> GSHMADPDVLTEVPAALKRLAKYVIRGFYGIEHALALDILIRNSCVKEEDMLELLKFDRKQLRSVLNNLKGDKFIKCRMRVETAADGKTTRHNYYFINYRTLVNVVKYKLDHMRRRIETDERDSTNRASFKCPVCSSTFTDLEANQLFDPMTGTFRCT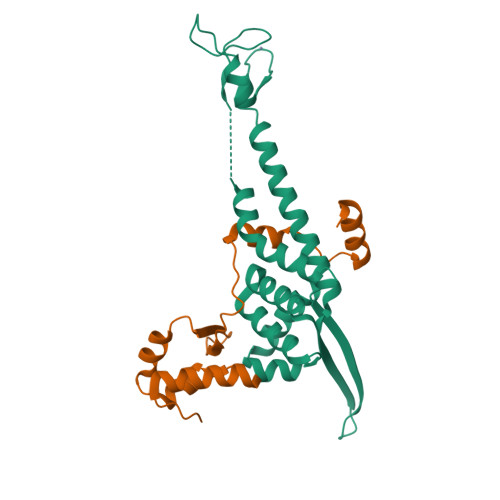FCHTEVEEDESAMPKKDARTLLARFNEQIEPIYALLRETEDVNLAYEILEPEPTEIPALKQS;> GSHMPKYNVRDKKALLRLLDQHDQRGLGGILLEDIEEALPNSQKAVKALGDQILFVNRPDKKKILFFNDKSCQFSVDEEFQKLWRSVTVDSMDEEKIEEYLKRQGISS>MGSSHHHHHHSSGLVPRGSMSLLFSPYQLGSLSLANRLVIAPMCQYSAVDGIAQDWHLMHLGRLAISGAGLVIVEATGVNPEGRITPFCLGLYNDEQEAALGRIVAFAREFGQAKMAIQLAHAGRKASTRRPWDPGSPYSPEEGGWQTWAPSAIKFYEESLTPHPMSIEDLETVKQDFVNSAIRAERAGFKAIELHGAHGYLIHQFLSPLSNQRQDQYGGSLENRMRYPLEILSAVKHALSAEMVVGMRISAVDWAPGGLTIEESITFSQECEKRGAGFIHVSTGGLVAHQQIPVGPGYQVEHAQAIKQNVNIPTMAVGLITHSAQAETILKSEQADMIAIARAALKNPHWPWTAALELGDKPFAPPQYQRAR[4x]

Old Yellow Enzymes (OYEs) are a broad family of flavoproteins with a modified TIM‐Barrel fold, adapted for the binding of the 5′‐phosphate of the FMN. These enzymes catalyze the reduction of a broad range of unsaturated carbonyl and nitrocompounds, creating stereocenters with high degrees of stereoselectivity. The reaction occurs through a ping‐pong mechanism, with a reductive and an oxidative half‐reaction. In 2017, Scholtissek et al. isolated a new OYE from the acidophilic iron oxidizer Ferrovum sp. JA12. This enzyme (FOYE), belonging to Class II OYEs, was thoroughly characterized, and despite coming from a mesophilic bacterium, it displayed an unusual thermal stability.

FOYE exhibits a tetrameric quaternary structure in the crystal with four molecules in the asymmetric unit. The electron density for the FMN is clearly visible in all the protomers, indicating good retention of the cofactor throughout the purification process. Since the reservoir solution contained a mix of lanthanides, we decided to place yttrium ions (depicted in cyan) at these positions. The four protomers are virtually identical, and, as for the other tetrameric OYEs, FOYE can be considered as a dimer of functional dimers (AB and CD, depicted in orange and lilac, respectively). Using the topological map of Yqjm as a reference [34], the tetramerization interface arises from the barrel helixes H6 and H7 and part of the loop L6. A small distortion of the helix H7 reduces the distance from the respective counterpart of the other protomer, allowing the formation of a π–π stacking interaction between the histidine residues H304 and a hydrogen bond between S314 and Q316. Notably, FOYE has a unique Q286–Q286 interchain hydrogen bond; in the other enzymes, these residues correspond to E270 and R300, which are in the range to form a salt bridge; however, in the crystal structures of TOYE and GkOYE, they appear with alternative conformations or form intramolecular salt‐bridges. The enzyme displays the signature C‐terminal α‐helix at the dimerization interface, which bears the typical arginine finger (R352) forming part of the other protomer's active site pocket. Moreover, as in the other Class II members, the threonine residue that interacts with the N5 and O4 of the FMN in Class I OYEs is substituted by a cysteine residue (C25 in Figure 4a). Differently from the other tetrameric OYEs, FOYE displays an extended unstructured region in loop L3 (residues 102–149), which is instead found in the other Class II enzymes, although with no homogenous length.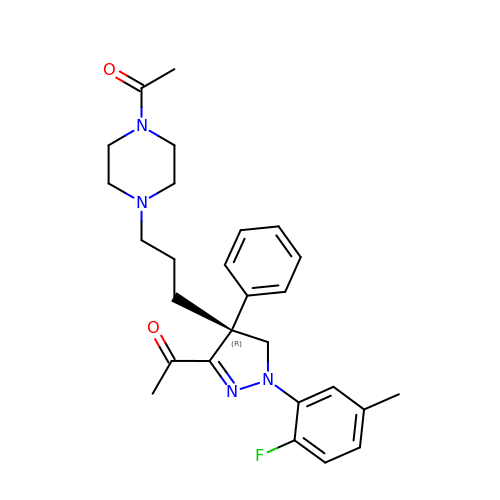1-[(4R)-4-[3-(4-ACETYLPIPERAZIN-1-YL)PROPYL]-1-(2-FLUORO-5-METHYLPHENYL)-4-PHENYL-4,5-DIHYDRO-1H-PYRAZOL-3-YL]ETHANONE | C27 H33 F N4 O2 | RYUBEOMELHCHMO-MHZLTWQESA-N> GPLGSNNELMPHGVKTKACVAGVDQAHCSVESKCYYTSISGSSVVAAITSSNPNLKVASFLNEAGNQIYVDLDPPCKF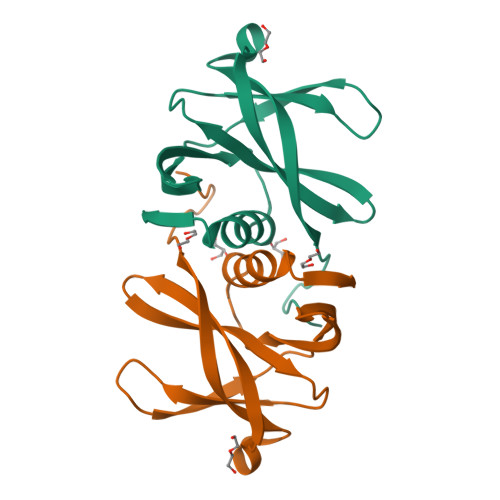GMKVGDKVEVVYLYFIKNTRSIVRGMVLGAISNVVVLQ>[4x]GPPTFNPPVPYFGRLQGGLTARRTIIIKGYVPPTGKSFAINFKVGSSGDIALHINPRMGNGTVVRNSLLNGSWGSEEKKITHNPFGPGQF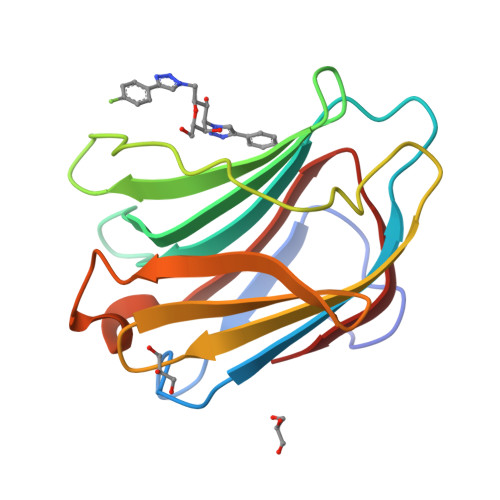FDLSIRCGLDRFKVYANGQHLFDFAHRLSAFQRVDTLEIQGDVTLSYVQI> MSDHGDVSLPPEDRVRALSQLGSAVEVNEDIPPRRYFRSGVEIIRMASIYSEEGNIEHAFILYNKYITLFIEKLPKHRDYKSAVIPEKKDTVK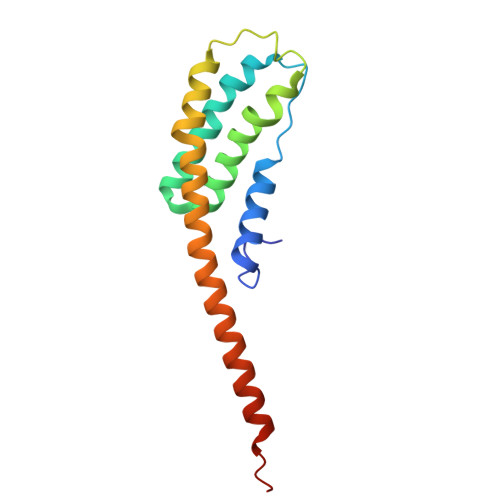KLKEIAFPKAEELKAELLKRYTKEYTEYNEEKKKEAEELARNMAIQQELEKEK> GSHMASMATGSEASKAAEAVVDWHKHDSKRMLHAVYRVGDLDRTIKYYTECFGMKLLRKRDVPDEKYTNAFLGFGPENTNFAVELTYNYGVDKYDIGTGFGHFAIANDDVYKLAENIKSKGGKITREPGPVKGGSTVIAFAQDPDGYMFQLIQRADTPEPLCQVMLRVGDLERSIKFYEKALGMKLLRKKDVPDYKYTIAMLGYADEDKTTVLELTYNYGVTEYSKGNAYAQVAIGTNDVYKSAEAVDLATKELGGK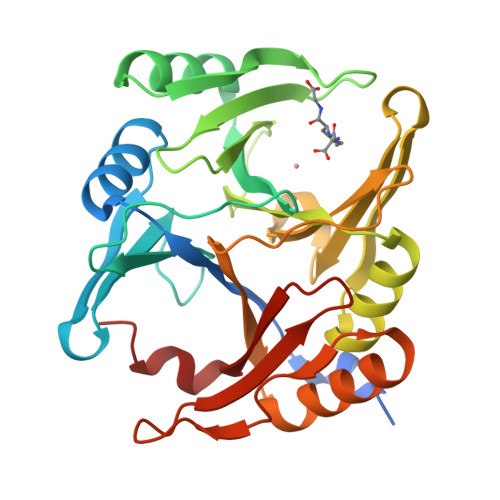ILRQPGPLPGINTKIASFVDPDGWKVVLVDNTDFLKELH> MFSLPTLTSDITVEVNSSATKTPFVRRPVEPVGKFFLQHAQRTLRNHTWSEFERIEAEKNVKTVDESNVDPDELLFDTELADEDLLTHDARDWKTADLYAAMGLSKLRFRATESQIIKAHRKQVVKYHPDKQSAAGGSLDQDGFFKIIQKAFETLTDSNKRAQYDSCDFVADVPPPKKGTDYDFYEAWGPVFEAEARFSKKTPIPSLGNKDSSKKEVEQFYAFWHRFDSWRTFEFLDEDVPDDSSNRDHKRYIERKNKAARDKKKTADNARLVKLVERAVSEDPRIKMFKEEEKKEKERRKWEREA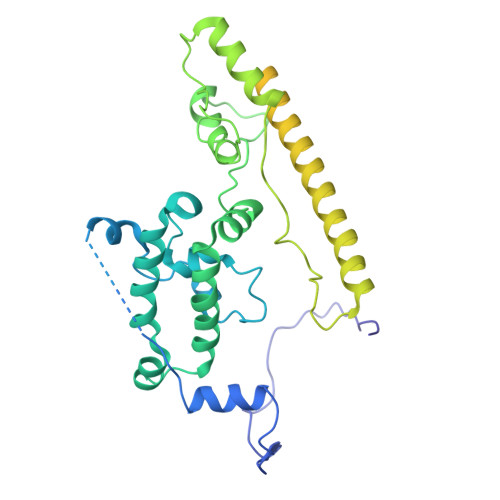GARAEAEAKAKAEAEAKAKAESEAKANASAKADKKKAKEAAKAAKKKNKRAIRNSAKEADYFGDADKATTIDEQVGLIVDSLNDEELVSTADKIKANAAGAKEVLKESAKTIVDSGKLPSSLLSYFV> MKQIVTINLNHICPMVTGVTPHIGGPIIGPGCPGVMVNGVPISVMGDMCVCCGPPDTIVQGEPGILVNGKPIVLQGCMTAHGGIIPAGVPGVTVSSASPIEPITMNHVSPKRNRFLAAISGNNLQEAIENQNALQKKMLEEEPMIFNVHWEKEDIHIAESHINKKVTVNADTIGFKDGE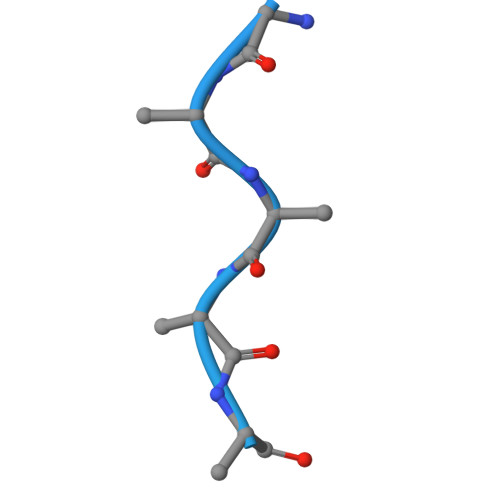TVKFVITPEAIDTANGEQVEDIELTGTVNNNHVTVEWIVELKK>GSHMGVGSVAALLTVVFYIAAVMATNLYGATFPEWFGDLSKSLYTLFQVMTLESWSMGIVRPVMNVHPNAWVFFIPFIMLTTFTVLNLFIGIIVDAMAITKEQEEEAKTGHHQEPISQTLLHLGDRLDRIEKQL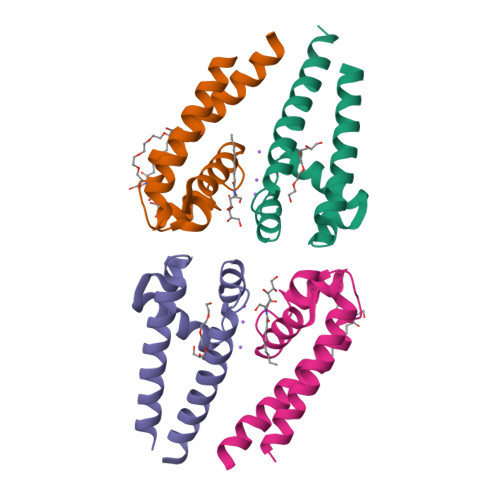AQNNELLQRQQPQKK[4x]>[3x]MHYAEAATPAKSAGSAVAKKHLEAKQKIGFVHGIDGTIATIAPAASKVTVPYNTVLEIAVSATNIANALVFNLEKDGSIGVILLDNISEVRSGQDVYATGSLLKIPVGFHMLGKIINPLGKEIPTGLFTKAAPLLDDTKLGLVEEMAPNIVSRQPVNYNLLTGYKVIDTLIPVGRGQRELILGDRQTGKTSIALSTILNQTKVNNEILSKNNVLSVYVSIGQRCSNVARIHRLLTEYDAMKYCTIVAATAADPAGLQYLAPYAGTTLGEEFRNSGRHILLVYDDLSKQAVSYRQISLLLRRPPGREAYPGDVFYLHSRLLERSAMMSPQKGSGSLTSLPIVETLSNDVTAYIVTNVISITDGQIYLDAKLFTGGQRPAVNIGLSVSRVGSSAQNKAMKKVGGALKMLMGEYRKMAGEQTSGSQNVSPVMIRGARCLQLFNQKGPSYFMDAIVALYAVTNGYMDDVKLQYSKFYEFLLLNKDLPVLYGQVNNKYFYMYNKNLNYFIRYFGLNHEILEPELKKYIEIHTNLFLDNYQSRMNELKSDEDLVQLKNLLYACKRTV;>[3x]TAPATAADVKQVGYVQQIIGAVVDVTFTDSVPPVLTALTVDAKETGTLLTMEIVQHLDTKTARCICMSSTDMLRLRTPVVNTGSQITVPVGEATLGRIFNVMGDAIDQRGPVKNKVRWPIHRKAPTLAEQSGKDEVLVTGIKVIDLILPYCKGGKIGLFGGAGVGKTVIIMELINNVAKGHGGYSVFAGVGERTREGTDLYLEMMGSKVIDLQGDSKCVLVYGQMNEPPGARARVAQTALTMAEYFRDEAGQDVLLFVDNVFRFTQANSEVSALLGRIPAAVGYQPTLAEDLGMLQERITSTVKGSITSVQAVYVPADDITDPAPATTFSHLDATTVLSRSVAEAGIYPAVEPLECASRIMDPDAIDVNHYNVAMDIVEMLTKYKELQDIIAVLGIDELSEEDKLIVDRARKVAKFMSQPFAVAEVFTGMKGYYVQLEDCVSDFGSLLMGQCDNIPEMAFYMVGGLDSVKEKAAKMAAEAAAMRERARKAAEAK;> MPGGGTIRFWREKLEGYKKYHQIVKTIKMVTLAKYRQTVVRTRVRDQTLRYTRKALDAKTQDDQEVIEKSECLLYVPITTNRGSCGALNTNMVRYLQEVENPKMTIISVGKKALDAMTKVFQDTYRRTILNDMKQAMSFQFAAYVLEHMNTVPWDRAQIVYNRYHGAASQKLAIFNLPKFEDWKQKLEEDSAGDGKIEEDGLLQSLPMKTALGELEETAVEDFYNFHSCLAVLNAVSENELSEYAARIVAVENQLGNITGLMQLADYTYNKTRKELITAELLEIIGTMTAMHAGKKVGLKKTEFWK;> MRASRTLLLSVSRFMRQDPRKFFPDNGFRFFDGPEDSFGDGNIPAQIILTLTRQDEFILKQEPVAAITIRTNEGEMGVLAGHEYTVQQLAPGILEVEYEGGKKDQYVISGGFAHVNDTGVVDINTVEAVPLEEIDHEKLAKALEEARAKSQSPDEAVRIQGEIALEIFEPLEAALH;> MSWRDAGISYLRYLSIVTRCIHEVQKEGPLLTKNVRFSTIGWKSLYLDHGATKEYTAIPAELEKIPENQVAQQHHA;>[3x]MQKLSRVVCNRLVRFHGTVAASAGGKRYDLFGYEVSVATGPFIEEIKKAQFYDDAGEVIVKMNLANTPPDLQTYNAVLERILNCKSKRSQPVKGENKFAAMMDILEEMDARSGIKPNAESWGYVLKELVQAGDFRLGWVCIAGMKSLGITPDQALVDANEANAAKAKAAGTDFPAYLKKAAPESFDTKAWGI;> MHMRRAVSVFGRCRSLNGLRNYAVPSPKYIEIYQSDFSRNAYPLELLGGSHVDFAKLLYSFADQVENKKFEVYVEDFKKLDSIIAEKGPFWAEEKIFQSPTFQGLSEGFKFILGWIQSEGAIDRLENVRLAYKELVNEARKETTATVIVAKEPSGNDLAEIRKQVEELHKESPLKDYKLVLETKVDPSIGGGYILEVCNQVVNRSAAAAAAETAALAKASAAQVDWTSLPAAPPRPSPSAPDTLIRLLGSVVDDLADADKVEQKYGA;>MQRGSSITKVVRRAALARSTRNAAIAYEVTVNGANLIGAGMAASGVGVPAIGVAMCFSSYMLAAARQPNMSAKLLPYCILGFALSEALALFTLLIALLELFVFS[10x]

The mitochondrial ATP synthase is a membrane protein complex that generates most of the ATP in eukaryotic cells. The translocation of protons through the membrane-bound Fo part, mediated by subunit a, drives the rotation of a membrane-embedded c-ring and the attached central stalk, which together form the rotor. The torque of the rotor against the stator subunits induces conformational changes in the (αβ)3 headpiece, thereby triggering catalysis. To reveal how the mitochondrial ATP synthase is modulated by lipids and organised into a dimer shaping discoid cristae in Euglenozoan mitochondria, we determined the structure of the ATP synthase dimer from E. gracilis.

Symmetry expansion of the pseudo-C2-symmetric dimer particles was used to classify individual F1/c-ring monomers into rotational states 1, 2 and 3 (named according to bovine nomenclature; Zhou et al., 2015) and resolve structures at 3.0- to 3.9 Å resolution. The E. gracilis F1/cring maps of rotational states 1 and 2 showed strong density for IF1, but weak density in rotational state 3. Subsequent focused classification of the IF1 binding site suggested complete inhibitor binding for rotational states 1 and 2, whereas rotational state 3 displayed a mixed occupancy, with a minority (34%) of particles containing IF1 and a majority (66%) not containing the inhibitor. Unlike the bovine ATP synthase, which displays a nearly equal particle distribution among the three rotational states, rotational state-3 (20%) is less populated than rotational states 1 (44%) and 2 (36%). Rather than reflecting dwell times during rotary catalysis, the distribution of rotational states is likely dictated by accessibility of the respective catalytic interfaces to IF1 binding, which for rotational state-3 may be sterically hindered by the proximity to the peripheral stalk. We observe this contact in all three rotational states, which provides the first observation of an interaction between the peripheral and central stalk in the ATP synthase. The position of the lumenal H5EG1 on the c-ring β-barrel remains largely unchanged in all three rotational states, suggesting a mechanism of transient rotor-stator interaction during c-ring rotation.In this study we showed that the CYTH enzyme in crenarchaeote S. acidocaldarius previously annotated as adenylyl cyclase is actually a phosphohydrolase of the TTM family. SaTTM prefers inorganic triphosphate substrate over NTPs. The general topology of SaTTM is described by an eight-stranded β-barrel comprising the antiparallel strands β1-β9/β5-β4-β3-β2-β6-β7-β8(-β1) with three interspersing α helices and the C-terminal plug helix α4. The enzyme formed a dimer in solution corresponding to 56 kDa compared with standards.

Initial attempts to produce diffraction quality crystals using apoenzyme were unsuccessful, but crystallization was finally possible under a high-sulfate condition. SaTTM was crystallized as an open-state homodimer, bound with two sulfate anions instead of the ATP that was included in cocrystallization. The open state of SaTTM was crystallized in space group P41212 with one monomer per asymmetric unit. The polypeptide is defined by electron density for R6-A176 but lacks completely residues P44-R49 and Q73-R80 due to missing density. The dimerization of SaTTM was also found in the crystal structure formed by two symmetry mates along the α2 helices and parts of the preceding β5 strand. PDBePISA revealed that the dimer interface covered 875 Å2 with a CSS score of 0.32 and accounts for 8.5% of the total solvent-accessible area of one protomer. The dimerization is mainly established by hydrophobic interactions of residues from β3, β4, β5, and α2 and salt bridges between K99 from one protomer and E81 from the other protomer. The C-terminal α4 plug helix blocks the tunnel entry from one side.

> MGSYIEREIKLRVISPSLEEIEERIRNNYTFINEEHQIDIYYNNPIRDFRKSDEALRLRNTNGKVILTYKGPKQSKETKTREEIEVEVSDLHKMDLILRKLGFIRSFQVEKIRKNYKYADFIISLDSIKELGEFIEIEGINKTEKELISFVDEFVKKHQIQYEKTIKSYLELLVEHAKKTNNSNTHGSIEGRHHHHHH> APSNSVPLTPLNSRQYSEDLAERQSWLLDQAKGLRSKYAPHLGERGQELRRRDIIDEGITRRKRANQKRATGTVSLTDVGLDASYAGQVSIGTPAQDFLVIMDSGSSDLWVAGSTCTENFCKQTYTFDTSTSSSFITSSEAFNITYGSGDADGTLGTDTVSMAGFTVSDQTFGVVTSTSANLISYPLSGLMGLAWKSIASSGATPFWQTLAASGDWDSPEMGVYLKRYRGDNTASQIETDGGQILFGGLNTSLYNGSVNYISIDESEKDYWRIPLEAMVIQGNSVSIASSSGGSN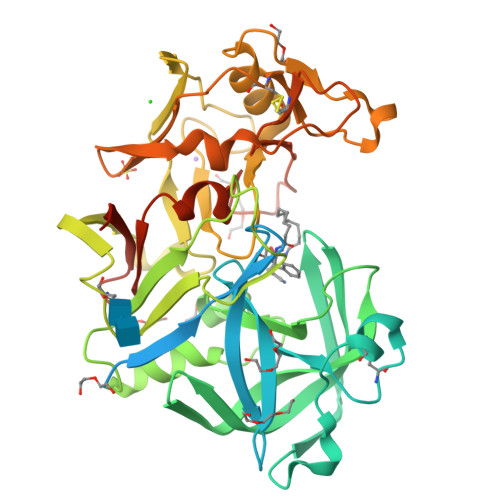PSCAIDTGTTLIGVPSQTANRIYSQIAGAEALSASSGYEGYYQYPCDTEVTVSLQFGGMSYSISNADMNLGSFTRDTSMCTGAFFAMDMSSRSPVQWIVGASFIKNVYTAFRYNPAAIGFAELAAAGLNDIFEAQKIEWHE To investigate protein HHP adaptation, Elastic Incoherent Neutron Scattering (EINS) and Quasi-Elastic Neutron Scattering (QENS) have been employed to study the dynamics of two orthologous proteins from T. barophilus (Tba) and T. kodakarensis (Tko), which only differ by their optimal growth pressure. X-ray crystallography was performed to obtain the structures of the proteins. Both present very similar features: their structure is dominated by β-sheet contributions with turns and disordered regions connecting them, forming a jelly-roll barrel structure, and both present a dimeric quaternary structure. The active site is located in a pocket inside the barrel and is conserved between the two proteins (His44, His46, Glu51 and His85). The two orthologs differ at 16 positions, and most of the substitutions are located at the protein–water interface and involve mainly polar and charged residues, with the notable exceptions of I35V, located in the hydrophobic core of the protein, and I100V, located at the monomer–monomer interface.

Interestingly, the catalytic metal ion coordinated by these four residues is found to be magnesium in Tba PMI and zinc in Tko PMI; however, the structure’s resolution does not allow for making a definitive assignment, as the Van der Waals radius of both ions is smaller than the resolution. Tba PMI crystals were obtained after two weeks from condition F7 of the Morpheus kit (Molecular Dimensions), containing a 0.12 M monosaccharides mix, 0.1 M buffer system 2 pH 7.5, 30% v/v precipitant mix 3. Tba PMI crystals belong to the I222 space group and contain one molecule in the asymmetric unit, while Tko PMI crystals belong to the P31 space group and contain eight molecules in the asymmetric unit. After model building using Coot and Refine from the Phenix package (Tba PMI) or REFMAC5 (Tko PMI), the final structures exhibited an R(%)/R(%)free of 0.18/0.20 at 1.7 Å (Tba PMI) and 0.23/0.29 at 2.2 Å (Tko PMI). The results show that the mechanisms by which Tba PMI counteracts the effect of HHP are: (i) the prevention of excessive amounts of water from penetrating the solvent-accessible cavities and limiting their destabilization, (ii) the inhibition of protein–water cooperative relaxations, and (iii) the reduction of internal (i.e., inaccessible to the solvent) cavity volume. To this extent, the I35V substitution appears to be key in the stabilization of the hydrophobic core, with the added importance of being close to the ligand pocket, limiting its deformation under extreme conditions. In the dimer-forming region, the I100V substitution optimizes the contact between the two monomers and decreases internal cavity volume, stabilizing Tba PMI’s quaternary structure under extreme conditions and seemingly maintaining optimal functionality.

> MKAEIKEFIDRGTYRKAPLFEGELPEGSYAQIVEIKPKQTVPKHYHEKQYELFYIISGQAKLGIEEREYDAKPGDIFLVKPKTVHWVVNKKEEPFRLFVIKLNYFGDDSVWLE>MTHYDVVVLGAGPGGYVAAIRAAQLGLSTAIVEPKYWGGVCLNVGCIPSKALLRNAELVHIFTKDAKAFGISGEVTFDYGIAYDRSRKVAEGRVAGVHFLMKKNKITEIHGYGTFADANTLLVDLNDGGTESVTFDNAIIATGSSTRLVPGTSLSANVVTYEEQILSRELPKSIIIAGAGAIGMEFGYVLKNYGVDVTIVEFLPRALPNEDADVSKEIEKQFKKLGVTILTATKVESIADGGSQVTVTVTKDGVAQELKAEKVLQAIGFAPNVEGYGLDKAGVALTDRKAIGVDDYMRTNVGHIYAIGDVNGLLQLAHVAEAQGVVAAETIAGAETLTLGDHRMLPRATFCQPNVASFGLTEQQARNEGYDVVVAKFPFTANAKAHGVGDPSGFVKLVADAKHGELLGGH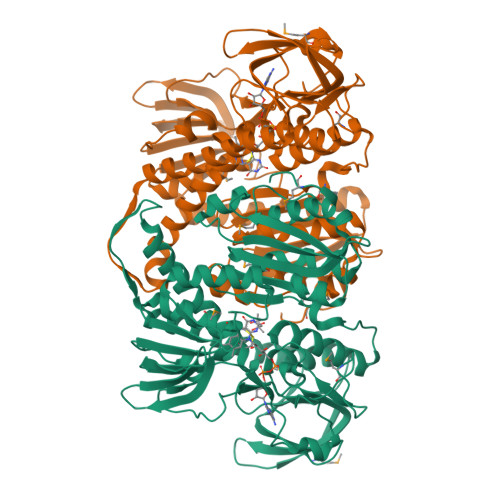LVGHDVAELLPELTLAQRWDLTASELARNVHTHPTMSEALQECFHGLVGHMINF[2x]1-(1H-imidazol-1-yl)ethan-1-one | C5 H6 N2 O | 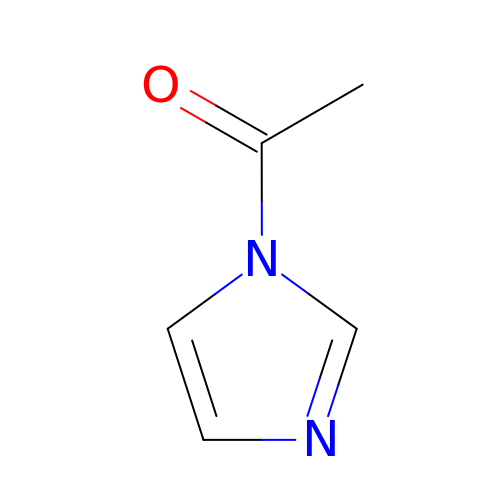VIHYIVKEECZGOU-UHFFFAOYSA-N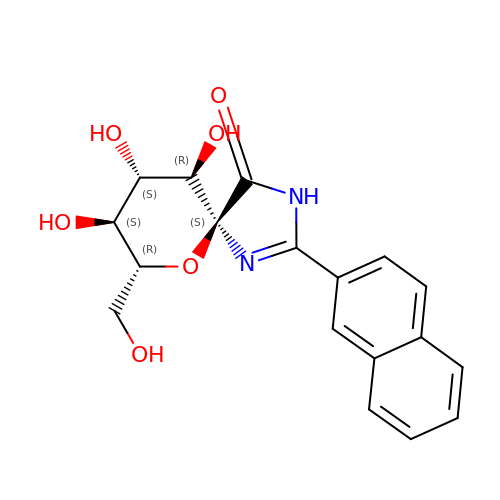(5~{S},7~{R},8~{S},9~{S},10~{R})-7-(hydroxymethyl)-2-naphthalen-2-yl-8,9,10-tris(oxidanyl)-6-oxa-1,3-diazaspiro[4.5]dec-1-en-4-one | C18 H18 N2 O6 | QSYAFZZRALZDHF-NSIVTLKISA-N2-[[(2~{R},3~{S},4~{R},5~{R})-5-(6-aminopurin-9-yl)-3,4-bis(oxidanyl)oxolan-2-yl]methyl-[3-[6-azanyl-9-[(2~{R},3~{R},4~{S},5~{R})-5-[(3-azanylpropanoylamino)methyl]-3,4-bis(oxidanyl)oxolan-2-yl]purin-8-yl]prop-2-ynyl]amino]ethanoic 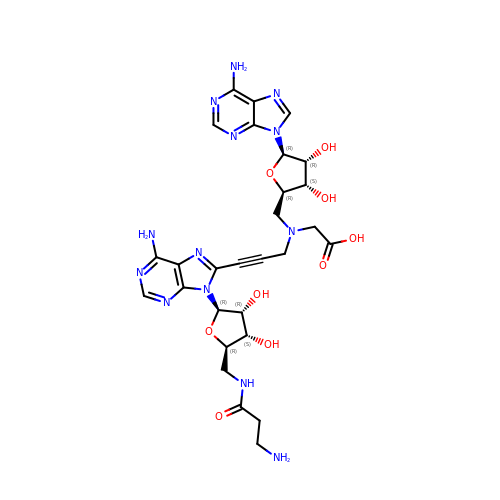acid | C28 H35 N13 O9 | MESAVOLQOCRHDN-QJYUSYPVSA-N>MVRPSQSMYDRHLTIFSPDGNLYQIEYAIKAVKNTNITSVGVKGENCAVIISQKKMATQYISQDKLLDYNNITNIYNITDEIGCSMVGMPGDCLSMVYKARSEASEFLYSNGYNVNAETLCRNICDKIQVYTQHAYMRLHACSGMIIGIDENNKPELFKFDPSGFCAGYRACVIGNKEQESISVLERLLEKRKKKIQQETIDEDIRNTTILAIEALQTILAFDLKASEIEVAIVSTKNRNFTQISEKEIDNYLTYIAERD[2x];>MADGEYSFSLTTFSPTGKLVQIEYALNRVSSSSPALGIRAKNGVIIATEKKSPNELIEENSIFKIQQISEHIGIVYAGMPGDFRVLLKRARKEAIRYSLQYGSEILVKELVKIIASIVQEFTQTGGVRPFGLSLLICGVDVYGYHLYQIDPSGCYFNWMATCVGKDYQNNMSFLEKRYNKDIEIEDAIHTAILTLKESYEGVLNEKNIEIGVAYDNKPFKILTQNEIKDYLIEIE[2x];>[2x]MARRYDSRTTTFSPEGRLYQVEYALEAINNASITIGLITKDGVILGADKVFISKLIDKANNYEKIYKIDKHIFCGVAGLNADANILINQSRLYAQRYLYNYNEVQPVSQLVVQICDIKQSYTQYGGLRPYGVSFLIGGYDTKDGYQLYHTDPSGNYSGWFATAIGTNNLTASSVLKQEWKNDMTLEEGLLLALKTLAKSTDTEIPKSEKIELAYLTNKDGEVYQKYLTEKEIEELIKLYTQKYIKE;>MSYDRAITVFSPDGHLLQVEHALEAVKKGGCAVAIKSSNFAVLAVEKKNIPKLQNPKTTEKLIKLDEHNCLAFAGLNADARVLVNKTRLECQRYYLNMDEPAPVDYIAKYVAKVQQKFTHRGGVRPFGIATLIAGFKNNKEICIYQTEPSGIYAAWKAQAIGKNAKIVQEFLEKNYQENMEQKDCIFLALKAIFEVVELSSKNVEVALLTEKDLTFIEEQEINSMVELIDQERTKNNEQNE[2x];>[2x]MFSTRSEYDRGVNTFSPEGRLFQVEYALGAIKLGSTAVGICVNDGVILASERRISSTLIEKDSVEKLLSIDDHIGCAMSGLMADARTLIDYARVECNHYKFIYNENINIKSCVELISELALDFSNLSDSKRKKIMSRPFGVALLIGGVDKNGPCLWYTEPSGTNTRFSAASIGSAQEGAELLLQENYKKDMTFEQAEILALTVLRQVMEDKLSTSNVEICAIKKSDQTFYKYNTDDISRIIDVLPSPVYPTIDMTA;>[2x]MYRNLYDTDNIIYSPEGRLYQVEYASEAIKQGTCAVAIKSKDYVVVSGLKKCISKLSFPQEKIFKIDDYIGISMSGITSDAKVLTKFMQNECLSHKFLYNENINIESLVRSVADKYQKNTQKSSKRAFGVGLMIAAYHNEPCIFETRPNGSYFEYDALSFGARSHASKTYLEKNLHLFEECSLEELILHCLKALKCSLSSESELTISNTALAVVGKNHPWQEISSLQLEEYLSKVKMDAEQEQVEENVQNEANE;>[2x]MAGLSAGYDLSVSTFSPDGRLYQVEYIYKSINNNNTALCLECKDGIICCCINSNMDKNKMIKKNSYNRIYHVNNNIIITYSGFDGDARNIIDRARSEANTYYYNFHTNIPLHILVNRISLYIHAYTLYWHMRPFAASIIISSFNEKDKGDIYCIEPNGACYKYSGIVIGKNKEMFKTEIEKKDYKDINVRDAIEDIYKFILTSDDHMNKNNLQNLVNFSWICKESSYEFQNIHEEILTPALNKAVEYIEKLN;>[2x]TTIIGIIYDNGVMLACDSRTSSGTFISNKCSRKINRINENLYVCRSGASAHSQKIIEIIKHYCVSMKNENRKKGRFHEGETIYDETTYDEEIDIDSINYLDYNNNNDNNLVTKNKYFYEDKFNDYNPLVENVAHITKKIIYTNNNFLSCALIFGGYDKIKKQQLYAVNLNGSIIEKHDFAVSGSGSIYIQSYLQDKYKKFMTKKECFNLILNCVKYAMHNDNSSGGLIRIVNITKSFVEEFTVVNTQMNFQY;>TTICGLVCQNAVILGADTRATEGPIVADKNCSKLHYISKNIWCAGAGVAGDLEHTTLWLQHNVELHRLNTNTQPRVSMCVSRLTQELFKYQGYKVCAIVLGGVDVNGPQLYGIHPHGSSCLLPFTALGSGSLNAMAVLEAKYRDNMTIEEGKNLVCEAICAGIFNDLGSGGNVDICVITKDSYQHIRPYKEPNMRLYHLPHPTIYPKGTTPILSEKIEYIKKFISVEDA[2x];>MGSIYNYNGGCVLGMSGSNCVAIACDLRLGANTFTTVSTKFSKIFKMNNNVYVGLSGLATDIQTLYEILRYRVNLYEVRQDAEMDVECFANMLSSILYSNRFSPYFVNPIVVGFKLKHYVDEEGEKKVNYEPYLTAYDLIGAKCETRDFVVNGVTSEQLFGMCESLYVKDQDENGLFETISQCLLSALDRDCISGWGAEVLVLTPEKIIKKKLKARMD[2x];>MDTLIGLRGNNFVVLAADTYSI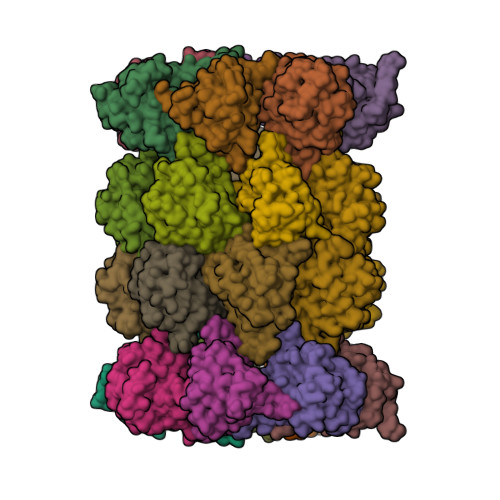NSIIKLKNDDNTKFYDIHGNKCLLLGGSIGDRLQFGEFIRKNVHLYQYQNNTDMFVKSFAFFTRKNLAYYLRRNPFEVNCLIAGYDKKDGYQLYWCDYLSNMDSVNKGAHGYGAYLVSAILDKYYHENLTVDEALDIFKLCFEELKKRFLLTQINYELRIMYDNKVETQYVTV[2x];>TTTLAFKFKDGIIVAVDSRASMGSFISSQNVEKIIEINKNILGTMAGGAADCLYWEKYLGKIIKIYELRNNEKISVRAASTILSNILYQYKGYGLCCGIILSGYDHTGFNMFYVDDSGKKVEGNLFSCGSGSTYAYSILDSAYDYNLNLDQAVELARNAIYHATFRDGGSGGKVRVFHIHKNGYDKIIEGEDVFDLHYHYTNPEQKDQYVM[2x];>MDLILYNDNLTEKKTEKENVIEHGRGFKRWYPYIDNGGTVIGLTGKDYVILAADTRLSLSYSIYTRFCPKISKLTDKCIIGSSGMQSDIKTLHSLLQKKIQLFVLEHSHYPDIHVIARLLCVILYSRRFFPYYAFNILAGVDENNKGVLYNYDSVGSYCEATHSCVGSGSQLILPILDNRVEQKNQLIKNTNFNLGDDINFVKDAITSATERDIYTGDKTLIYVIDKMGINVNTLDLKQD[2x];>MTLGPVVTGTSVIAIKYKHGIMIAADRKASYGSYAKFQNVERIFKINNKTVMGFSGELADAQYLHELLTRKNINNLSEKKRKEDMYTPQHYHSYVSRVFYVRKNRIDPLFNNIIIAGINSQKYDNNDDNVLLYTNKNNDDEQNEYKNNEEYKEIHKDDLYIGFVDMHGTNFCDDYITTGYARYFALTLLRDHYKDNMTEEEARILINECLRILYFRDATSSNFIQIVKVTSKGVEYEEPYILPCVLNSADYVYPSTLLPPAGCMW[2x]N1-CYCLIC INOSINE 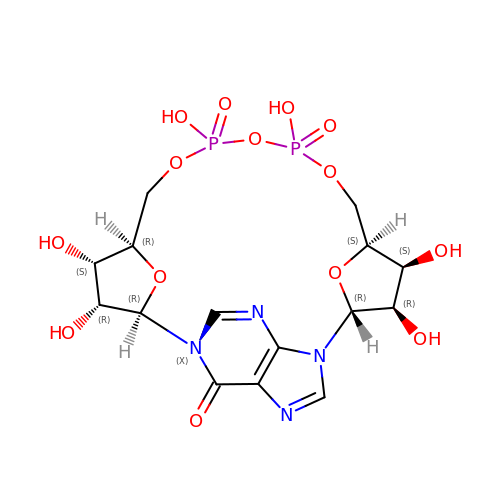5'-DIPHOSPHORIBOSE | C15 H20 N4 O14 P2 | REBZYOYBILSKBL-ATYUDWGKSA-N>[2x]MASENIEVHMLNKGAEGAMVFEPAYIKANPGDTVTFIPVDKGHNVESIKDMIPEGAEKFKSKINENYVLTVTQPGAYLVKCTPHYAMGMIAL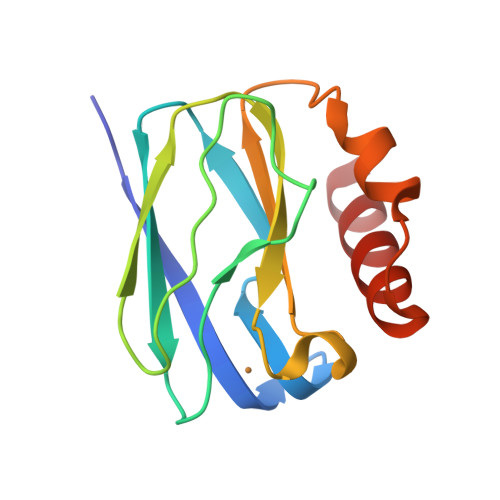IAVGDSPANLDQIVSAKKPKIVQERLEKVIASAK3-{3,5-DIMETHYL-4-[3-(3-METHYL-ISOXAZOL-5-YL)-PROPOXY]-PHENYL}-5-TRIFLUOROMETHYL-[1,2,4]OXADIAZOLE | 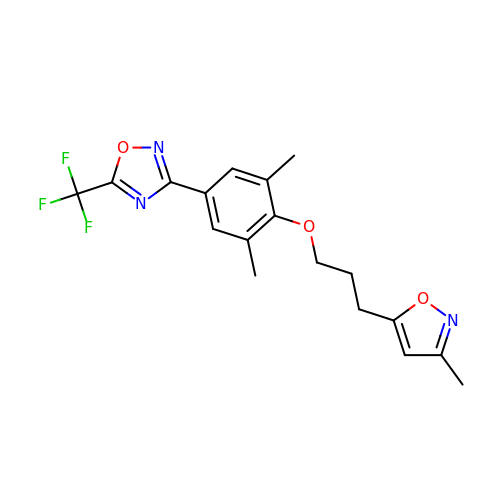C18 H18 F3 N3 O3 | KQOXLKOJHVFTRN-UHFFFAOYSA-N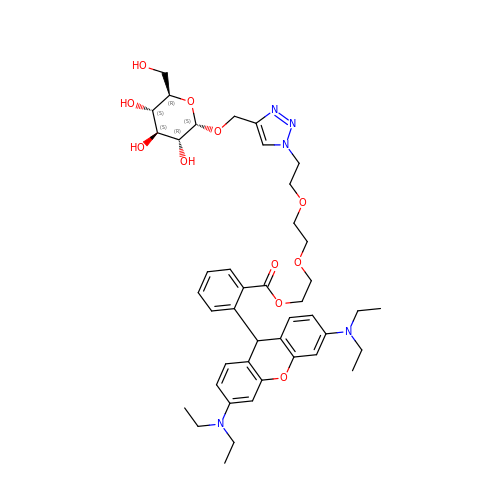2-[2-(2-{4-[(alpha-D-glucopyranosyloxy)methyl]-1H-1,2,3-triazol-1-yl}ethoxy)ethoxy]ethyl 2-[3,6-bis(diethylamino)-9H-xanthen-9-yl]benzoate | C43 H57 N5 O11 | LPSYXQPVOZLKRL-OUZFDYGBSA-N> MASSLGFGGSNAVDKVNATTTPGTVATPNSGPTKMLDEHILTPASISTLEVHGATNTRRSLLDQIFKPVLEDTAAAGTTLGQVLDRVGAATKKLARFDIFKEEGFGVFLSEAAPPQSAPPTDRTDLDISIRVKEKSRLVFSAGTDFGNAEGSAYTNAVVRNIFGGAETLTVNASTGTRTRSAYNATFSTPING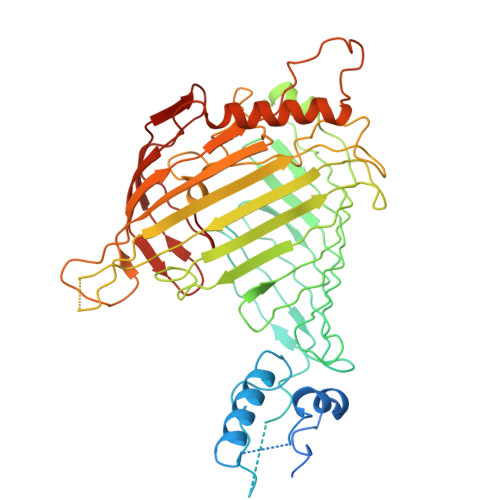NPDLRLSVEALRSATQKPWASHEEHLTGANLRLAWLTEKGDTHALAYSSVWRQLTGLAPTASPTVRADAGDSLKSSLTHTFTRDRRDNPMLPQSGYLFRSVSELAGWGPLNGDVSFAKTEVEASGALPVAIPGLAGKSGVSVGGGLRLGVLYPLPLGYSLTGAAQPSRINDRFQLGGPNDVRGFKIGGLGPHDGVDAVGGDVFAAGSVNALLPLPRTGPDSPLRLQLYANAGRLVALNSKGTDKEGKEGLAMDSAAVFKGVKSAVGKLTNGIPSLAAGVGLVYAHPVARFELNFSLPLVLRRGEEGRKGLQVGVGISFL>[4x]MSMAERKALCLEMVAAWNRWDLSGIIKHWSPDIVHYSEDNEVSSADMVKLMEGGLKAFPDLQLEVKSIMAEEDRVA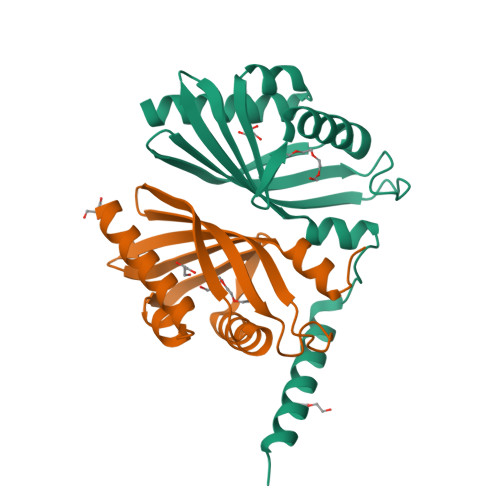LRITVTATHQGEFMGVQPTGQRVSWHLVEELRFVDGKVVEHWDVINMRPLLVRLGKLPDVPKVVLEASAKLAAALEHHHHHH Here, we take a structural approach to assess the relatedness of these eukaryotic-like proteins in Asgard archaea, the closest known prokaryotic relatives to eukaryotes. Asgard archaea roadblock, longin and TRAPPC3 domain-containing proteins form dimers similar to those found in the eukaryotic TRAPP and Ragulator complexes. Here, we adopted an X-ray crystallography approach to compare the structures of a potential Asgard Rab small GTPase, several RBs and two TRAPPC3 proteins to their eukaryotic counterparts, with a focus on Thor and MKD1. We conclude that the emergence of these protein architectures predated eukaryogenesis, however further adaptations occurred in proto-eukaryotes to allow these proteins to regulate distinct internal membranes.

Finally, we investigated the TRAPPC3-like proteins from Thor. The crystals were pink in color indicating potential Zn2+ binding. We further analyzed the homology around the Thor-TRAPPC3 Zn2+-binding site. We found that the predicted Zn2+-binding sites and the experimentally determined sites are not completely conserved in positions of the coordinating residues, rather they appear in similar regions and appear to serve the same function in tethering the β-sheet to the D α-helix to create cavities. Interestingly, mouse TRAPPC3 has evolved to replace the Zn2+-binding site by a hydrogen bond. We speculate that Thor-TRAPPC3 may also bind small molecules, potentially being involved in ligand transport. The cavities appear to be accessible from the exterior close to the dimerization interfaces. Furthermore, we uncover structural evidence that TRAPPC3-like proteins exist in several branches of Asgard archaea and are likely to share a common ancestor gene with the V4R-like domain.

>[4x]GPMPKVENPLLISLYSHYVEQILSETNSIDDANQKLRDLGKELGQQIYLNTEIVEKTKENVTTREEVAKLIENVYKVLFDKKPKDVDMKTARGSVRITDDNCVWCQEVNLEGMRGFGYCEIFSGILESILEFKGVDAKVFQEMSKATGSDVCVWNVRLV Here we describe a new mechanism by which foot-and-mouth disease virus (FMDV) can become resistant to ribavirin. Amino acid changes in the viral polymerase, selected by ribavirin, are able to modify the types of mutations produced in the presence of ribavirin. P44S but not P169S was detected in a 70% proportion in R-Ap35, as evidenced by analysis of both the consensus sequences and their corresponding mutant spectra. These results suggest that the three substitutions in 3D were selected sequentially during replication in the presence of increasing concentrations of R: first M296I, then P44S and finally P169S. To identify possible structural modifications of the viral polymerase associated with the important alterations of the mutational spectrum in progeny RNA, and to investigate how these modifications can affect RNA binding and polymerase activity, the different mutant 3Ds were incubated with the heteropolymeric sym/sub-U RNA of sequence 5′GCAUGGGCCC3′, crystallized, and analyzed by X-ray diffraction.

In contrast, 3D(SSI) crystallized in the trigonal P3221 space group with the sym/sub-U RNA incorporated in the structure. The X-ray structures were determined to 2.2 Å and 2.6 Å resolution for 3D(P44S) and 3D(P169S), respectively, and to 2.6 Å and 2.5 Å for 3D(P44S, M296I) and 3D(SSI), respectively. The analysis of the electron density showed also the presence of the duplex portion of the template-primer RNA in the central channel of the polymerase of the trigonal 3D(P44S, M296I) and 3D(SSI) crystals. The 3D(P44S, M296I)-RNA and 3D(SSI)-RNA structures are almost identical (rmsd of the superimposition of all polymerase residues of 0.22Å). However, the crystal structures of 3D(P44S, M296I) and 3D(SSI) in complex with the RNA template-primer reveal a rearrangement in the template channel with important effects in template binding, in particular, at position n+1 (nucleotide A3). The conformational changes in the main and side chains of residues M16 and R17 allow the opening of a hydrophobic pocket formed by residues of motifs G and F and by M16 that facilitates the entrance of nucleotide A3. In 3D(P44S, M296I)-RNA and 3D(SSI)-RNA complexes the re-oriented residue R17 points to the polymerase interior, interacting with the side chain of residues N41 (which lies in the same loop of the substituted amino acid S44), and with Y285. Nucleotide A3 appears also reoriented, flipped-out towards a pocket formed by amino acids M16, P117, G118, Q160, F162, V181 and V183. Interestingly, the incorporation of RMP opposite C was 3-fold lower for 3D(SSI) than for 3D(M296I), but no such difference was observed when the incorporation of RMP was measured opposite U.

> GLIVDTRDVEERVHVMRKTKLAPTVAHGVFNPEFGPAALSNKDSRLNEGVVLDEVIFSKHKGDTKMSAEDKALFRRCAADYASRLHSVLGTANAPLSIYEAIKGVDGLDAMEPDTAPGLPWALQGKRRGALIDFENGTVGPEVEAALKLMEKREYKFACQTFLKDEIRSMEKVRAGKTRIVDVLPVEHILYTRMMIGRFCAQMHSNNGPQIGSAVGCNPDVDWQRFGTHFAQYRNVWDVDYSAFDANHCSDAMNIMFEEVFRTEFGFHPNAEWILKTLVNTEHAYENKRITVEGGIPSGCSATSIINTILNNIYVLYALRRHYEGVELDTYTMISYGDDIVVASDYDLDFEALKPHFKSLGQTITPADKSDKGFVLGHSITDVTFLKRHFHMDYGTGFYKPVMASKTLEAILSFARRGTIQEKLISVAGLAVHSGPDEYRRLFEPFQGLFEIPSYRSLYLRWVNAVCGDAAALAHHHHHHH> PAGIIPTGNVLSTIEVCAHRCIFDFFKQIRSDDNSLYSAQFDILLGTYCNTLNFVRFLELGLSVACICTKFPELAYVRDGVIQFEVQQPMIARDGPHPVDQPVHNYMVKRIHKRSLSAAFAIASEALSLLSNTYVDGTEIDSSLRIRAIQQMARNLRTVLDSFERGTADQLLGVLLEKAPPLSLLSPINKFQPEGHLNRVARAALLSDLKRRVCADMFFMTRHAREPRLISAYLSDMVSCTQPSVMVSRITHTNTRGRQVDGVLVTTATLKRQLLQGILQIDDTAADVPVTVLNGANLVTALVMGKAVRSLDDVGRHLLDMQEEQLENARVPADLVIVGDKLVFLEALERRVYQATRVAYPLIGNIDITFIMPMGVFQANSMDRYTRHAGDFSTVSEQDPRQFPPQGIFFYNKDGILTQLTLRDAMGTICHSSLLDVEATLVALRQQHLDRQCYFGVYVAEGTEDTLDVQMGRFMETWADMMPHHPHWVNEHLTILQFIAPSNPRLRFELNPAFDFFVAPGDVDLPGPQRPPEAMPTVNATLRIINGNIPVPLCPISFRDCRGTQLGLGRHTMTPATIKA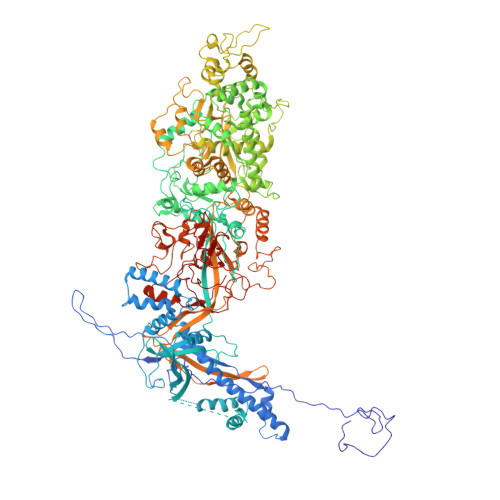VKDTFEDRAYPTIFYMLEAVIHGNERNFCALLRLLTQCIRGYWEQSHRVAFVNNFHMLMYITTYLGNGELPEVCINIYRDLLQHVRALRQTITDFTIQGEGHNGETSEALNNILTDDTFIAPILWDCDALIYRDEAARDRLPAIRVSGRNGYQALHFVDMAGHNFQRRDNVLIHGRPVRGDTGQAIPITPHHDREWGILSKIYYYIVIPAFSRGSCCTMGVRYDRLYPALQAVIVPEIPADEEAPTTPEDPRHPLHAHQLVPNSLNVYFHNAHLTVDGDALLTLQELMGDMAERTTAILVSSAPDAGAATATTRNMRIYDGALYHGLIMMAYQAYDETIATGTFFYPVPVNPLFACPEHLASLRGMTNARRVLAKMVPPIPPFLGANHHATIRQPVAYHVTHSKSDFNTLTYSLLGGYFKFTPISLTHQLRTGFHPGIAFTVVRQDRFATEQLLYAERASESYFVGQIQVHHHDAIGGVNFTLTQPRAHVDLGVGYTAVCATAALRCPLTDMGNTAQNLFFSRGGVPMLHDNVTESLRRITASGGRLNPTEPLPIFGGLRPATSAGIARGQASVCEFVAMPVSTDLQYFRTACNPRGRASGMLYMGDRDADIEAIMFDHTQSDVAYTDRATLNPWASQKHSYGDRLYNGTYNLTGASPIYSPCFKFFTPAEVNTNCNTLDRLLMEAKAVASQSSTDTEYQFKRPPGSTEMTQDPCGLFQEAYPPLCSSDAAMLRTAHAGETGADEVHLAQYLIRDASPLRGCLPL> MICLGLEGTAEKTGVGIVTSDGEVLFNKTIMYKPPKQGINPREAADH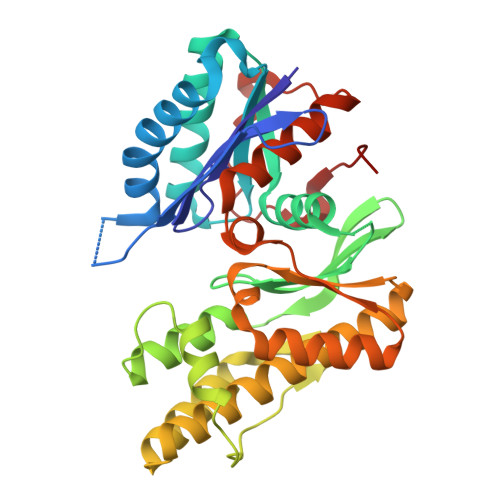HAETFPKLIKEAFEVVDKNEIDLIAFSQGPGLGPSLRVTATVARTLSLTLKKPIIGVNHCIAHIEIGKLTTEAEDPLTLYVSGGNTQVIAYVSKKYRVFGETLDIAVGNCLDQFARYVNLPHPGGPYIEELARKGKKLVDLPYTVKGMDIAFSGLLTAAMRAYDAGERLEDICYSLQEYAFSMLTEITERALAHTNKGEVMLVGGVAANNRLREMLKAMCEGQNVDFYVPPKEFCGDNGAMIAWLGLLMHKNGRWMSLDETKIIPNYRTDMVEVNWI o-cresol | C7 H8 O | 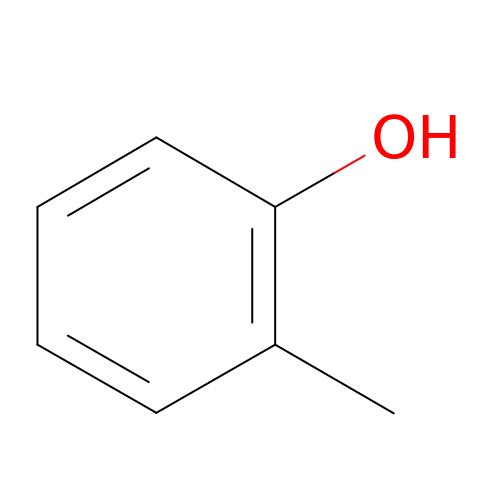QWVGKYWNOKOFNN-UHFFFAOYSA-N The primary mode of resistance to aminoglycoside antibiotics is through chemical modification catalyzed by aminoglycoside-modifying enzymes. Here we present the first structural and functional studies of two aminoglycoside-modifying enzymes that do not use target mimicry, AAC(3)-Ia and AAC(3)-XIa. X-ray diffraction studies reveal that these enzymes bind aminoglycoside antibiotics in a conformation where the central 2-deoxystreptamine ring is in boat conformation. Similar to other AACs, AAC(3)-Ia and AAC(3)-XIa display the GNAT superfamily fold.

In contrast, all five structures of AAC(3)-XIa contain both protomers of the physiological dimer in the asymmetric unit. Despite a tenfold molar excess of antibiotic to enzyme during crystallization, electron density maps of AAC(3)-XIa only allowed for the positioning of one aminoglycoside per physiological dimer. The experimental maps of the antibiotics in all AAC(3)-Ia and AAC(3)-XIa ternary complex structures presented in this report unambiguously place the aminoglycosides’ central ring in a boat conformation rather than the canonical chair conformation. Additionally, in all of these aminoglycosides the N-3, O-4 and O-5 atoms of the central ring were positioned in an axial plane rather than an equatorial plane, positioning the prime ring of aminoglycoside around 90° to the central ring. The shape of the pockets rationalizes these enzymes’ preference for 4,6-disubstituted aminoglycosides, as any hexose substituent at O-5 would provoke steric hindrance. In the AAC(3)-Ia and AAC(3)-XIa complexes, regions of the adjacent protomer in the swapped dimer contribute to the aminoglycoside binding sites. In the AAC(3)-XIa structure, the swapped dimer regions are folded closer to the aminoglycoside, creating a more enclosed pocket than is observed in AAC(3)-Ia. In AAC(3)-Ia, the aminoglycoside site is opened and easy for ligands to access, whereas in AAC(3)-XIa, the aminoglycoside binding site is closed off and the enzyme would require a conformational shift to accept reactants and release products.

>[2x]MTTTNEIRVAEVADAGVVAKLLRDFNTEFDTPVPEGLEERFAQIIAHDDAFVLLAGDIGFAYVTLRPSPYYDGPVAMLDELYVAPAHRNRGVGTALLQRVFEEIRKHSAGELQINVDEVDTDARRFYERHGLTNIEQGSRMLLYIREL> AMPLDAGGQNSTQMVLAPGASIFRCRQCGQTISRRDW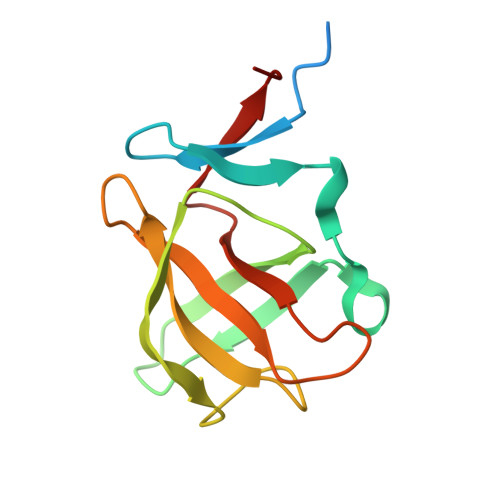LLPMGGDHEHVVFNPAGMIFRVWCFSLAQGLRLIGAPSGEFSWFKGYDWTIALCGQCGSHLGWHYEGGSQPQTFFGLIKDRLAEGPAD> EHYSVIQNSLNDKIVTISCKADTNLFFYQVAGNVSLFQQTRNYLERWRL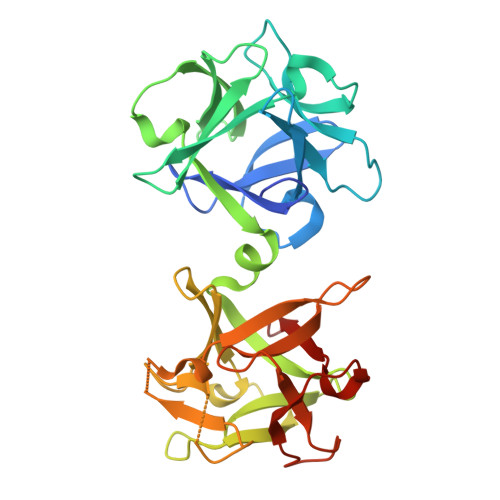IYDSNKAAYKIKSMDIHNTNLVLTWNAPTHNISTQQDSNADNQYWLLLKDIGNNSFIIASYKNPNLVLYADTVARNLKLSTLNNSNYIKFIIEDYIISDLNNFTCKISPILDLNKVVQQVDVTNLNVNLYTWDYGRNQKWTIRYNEEKAAYQFFNTILSNGVLTWIFSNGNTVRVSSSNDQNNDAQYWLINPVSDTDETYTITNLRDTTKALDLYGGQTANGTAIQVFNYHGDDNQKWNIRNPPGSA>GSHMSKKRQWALEDFEIGRPLGKGKFGNVYLAREKQSKFILALKVLFKAQLEKAGVEHQLRREVEIQSHLRHPNILRLYGYFHDATRVYLILEYAPLGTVYRELQKLSKFDEQRTATYITELANALSYCHSKRVIHRDIKPENLLLGSAGELKIADFGWSVHAPSSRRTDLCGTLDYLPPEMIEGRMHDEKVDLW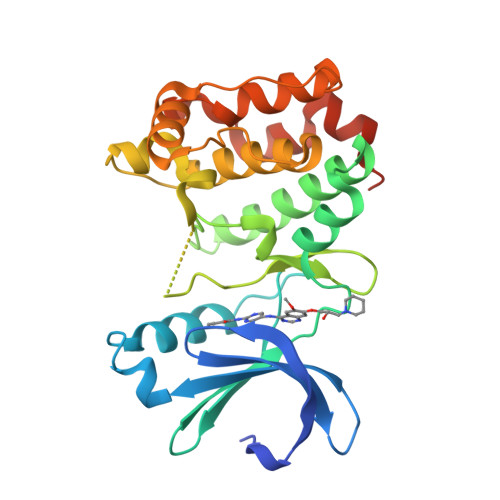SLGVLCYEFLVGKPPFEANTYQETYKRISRVEFTFPDFVTEGARDLISRLLKHNPSQRPMLREVLEHPWITANSSKPSNCQNKESASK[2x]>KFAEHLSAHITPEWRKQYIQYEAFKDMLYSAQDQAPSVEVTDEDTVKRYFAKFEEKFFQTCEKELAKINTFYSEKLAEAQRRFATLQNELQSSLDAQKESTGVTTLRQRRKPVFHLSHEERVQHRNIKDLKLAFSEFYLSLILLQNYQNLNFTGFRKILKKHDKILETSRGADWRVAHVEVAPFYTCKKINQLISETEAVVTNELEDGDRQKAMKRLRVPPLGAAQPAPAWTTFRVGLFCGIFIVLNITLVLAAVFKLETDRSIWPLIRIYRGGFLLIEFLFLLGINTYGWRQAGVNHVLIFELNPRSNLSHQHLFEIAGFLGILWCLSLLACFFAPISVIPTYVYPLALYGFMVFFLINPTKTFYYKSRFWLLKLLFRVFTAPFHKVGFADFWLADQLNSLSV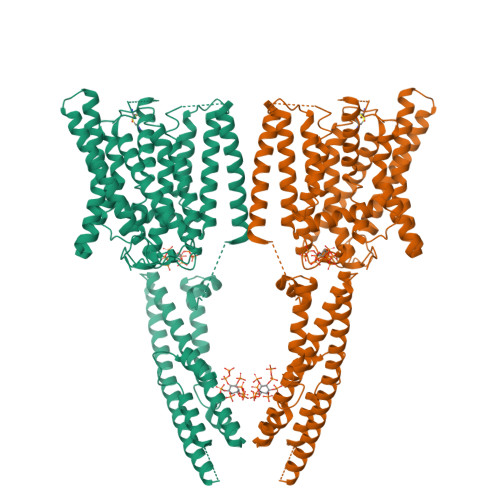ILMDLEYMICFYSLELKWDESKGLLPNNSEESGICHKYTYGVRAIVQCIPAWLRFIQCLRRYRDTKRAFPHLVNAGKYSTTFFMVTFAALYSTHKERGHSDTMVFFYLWIVFYIISSCYTLIWDLKMDWGLFDKNAGENTFLREEIVYPQKAYYYCAIIEDVILRFAWTIQISITSTTLLPHSGDIIATVFAPLEVFRRFVWNFFRLENEHLNNCGEFR[2x]> WRGSHHHHHHGSACASGKKDTTSGQKLKVVATN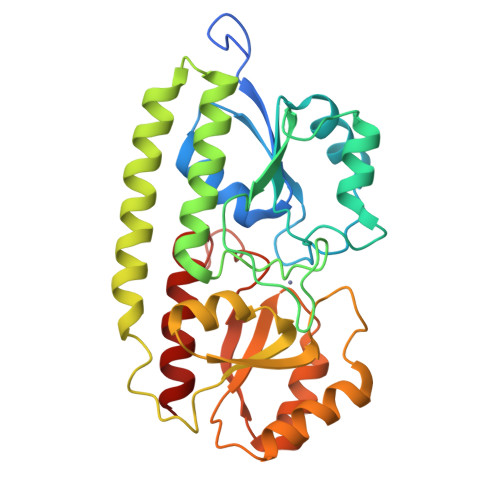SIIADITKNIAGDKIDLHSIVPIGQDPHEYEPLPEDVKKTSEADLIFYNGINLETGGNAWFTKLVENAKKTENKDYFAVSDGVDVIYLEGQNEKGKEDPHAWLNLENGIIFAKNIAKQLSAKDPNNKEFYEKNLKEYTDKLDKLDKESKDKFNKIPAEKKLIVTSEGAFKYFSKAYGVPSAYIWEINTEEEGTPEQIKTLVEKLRQTKVPSLFVESSVDDRPMKTVSQDTNIPIYAQIFTDSIAEQGKEGDSYYSMMKYNLDKIAEGLAK PHOSPHATIDYLGLYCEROL-PHOSPHOGLYCEROL | 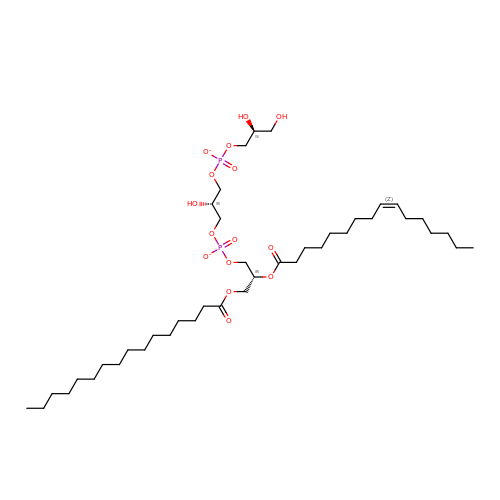C41 H78 O15 P2 | LXWNXFZWWXODAH-XOLIOQKMSA-L2-[1-(cyclohexylmethyl)piperidin-4-yl]-1-{3-[3-{[2-(4-fluoropiperidin-1-yl)ethyl]sulfanyl}-4-(trifluoromethyl)phenyl]-1-(3-hydroxypropyl)-1,4,6,7-tetrahydro-5H-pyrazolo[4,3-c]pyridin-5-yl}ethan-1-one 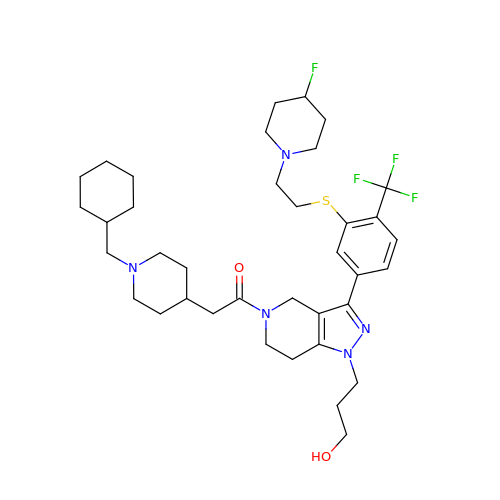| C37 H53 F4 N5 O2 S | HHMNMVKIYRQSRB-UHFFFAOYSA-N> MAMPR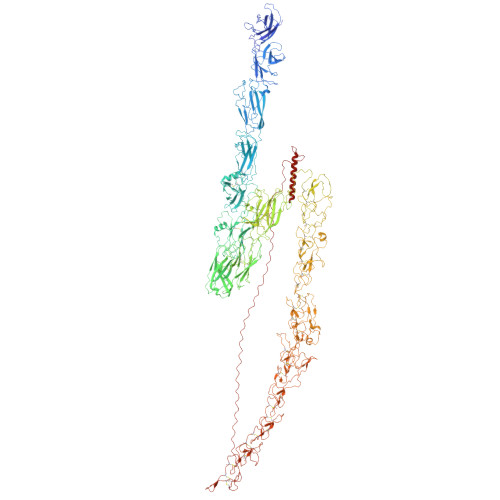HGRRPARCSSNRASQWLLLVLGVALAASPRFLLLVEAATYTLTLDKLGPTVNPTTSDAVTFTATVASPDSTTAVFFTLDYGDGVTAETTRTTTGALSTTPTANLVSAGTYTVTYASIGTKFVTLRLYDSAVAPGVLLASKTVPIYVEDSTLTATLLQSGVPRLNLAFSGFKGRVSSSTANRADMWATIQLDTAPGVFESSRIFIGIAPTASTNYDFVIPDQVYNLEGAKTTVLRIYDAPVGGTLLRTFTPAAANAVYVVDPSKYVLTLTVGPTSVTTADQVTFTQTTTEVSYSASATSPILQWRFNWDDPSVVETPLAYPDALTAASNFPTTATAVSSAAASTFRYTSTGSKNARLRLYDGANNVIAEKIVVITVSNAGYTLALAKTTADPVTTDDTIAFSAGAKHLSSTSQVWWTIDYGAGESSPRTALTMTNVGAAAPNAIASLSNQYTSGGTKLATLRIYDRDGVGANTGLLLASTTVTFTVTPVLYALESAVEPFSPIATVAAKWSFRIQRSKATPAGVTESIKCAFFGADTGTAPADLAAWLTAANGAGGLTATILPSSIPSDIISFTRTYAAAAASLQGKLQCFIGSTPLWDPYYPTPVFQVLAAAPTYTLSASVTPAVVPVDTATLWTYNIIRSVPVPAGGPSLPILCSFWDGKTGAAPTTDAGWAALAGSANGKGTSMAPGSTTATCSFTPSYSTTGTATPTLQLIQNSFALDAATTVGFLSPVYTAPAFATVTAASYTISSYLNPVTPVAGGAAAVWRIVITRNAAVTASAKTLTCQMPDNGQGGSPADVTADIAVGGTTTVCVFSIAGYTTATPGPYFATVNVVDGAVTTSHITKNFTVLASGTTAPTYAVTSVVSPATPVKVSTPVTYTFTITRTTAVPAGGIPQPIICEFFNGEGTAPASAAAYWRVSTTIPDADTVVAVMAPGETTTTCTFTTYYTTVSAGGFTAKLMVFGESATAAPLLTSLSVTPSQLLAAVHSFATPMVVAAAVVAVESTTISPNYNPTTPYTNIPTYFTFTLLRDPPVPPSASSGVQFACALYTGQNVNPASAPSAITDAVYKTFTDVTTAVATDANYFADQQLRVVTMAPGTGRVSCTFPTLYAAAGPFSPKFFVFEYASSTVGANALAVADTVTSLTSFTTQAAPTFITGPTNVPQRVPLPKGFRTTCFDGYELIFSNDNYTNGVRVAVDAYPYPVGQCRKCPGGTATMDGYRCIPCPSGYWSNEGARECTACPAGTIAKPAALTARAKYSIDPTTYHFVTHLAMGPESCKKCPKGYFQPNIAGTVCLPCPSGFVSTSGATGCTACSEGTYHTDGVGTTTPGEATSLDTTDTFGSIYPIIPNTCRQCPANTYLPLRGQAAIASMNLAAVSSATPCRPCEDGTWSKAGAAGCQKCPPGTYRNTWFSGQLGSPFITADGVPVATTLTELGSGCSQCPPGTYAPTFGMSVCLPCPAGTFASAPGATACQQCKPGTNSLMGDRTQQMALVVTNAANDFPALRAYTISGMVAGPAYAKPIVTGPDTNFFMAGKSETCSTNLPGYYTDVDGLPIQLPCKPGTFMPFDTATANLLDTGLTVDGTQCYTCQTGTFNDEFSQPVCKACWSGSFASKRGLPTCEIAQPGTFTNVAAAANATFNTATLIPTGLVKGAQAPTPCGMGYFQSSAETTTCTACAVGTYADQAGLAACKPCQPGRYQNSIGQRVCKPCDMGTYSRYGGELCTKCPAGTVASKTGSSQCTPCAAGFYANAPDSATSCRACPRGYYGPYSGAYADNLGDEFEGPRGCYKCPYDFFADRPGVRQCTACPPLDLGGGNLVEQCTEDLGSQRCKPCSLLSKPKTARTEQSPPPPSPSPPPPPPPSPRPPSPNPPSPRPPSPAPPSPNPPPTSPPPSPPPSPPPPRPPPPPPPPPSPPPPNRSPPPPPPASSAINPGGGVNQNGDPVGHRRAILSLMEDEDAEAAQEEQAIVDVDAEMQPQDDE> GPHMKHPLMNVWTLWYLENDRSKSWEDMQNEITSFDTVEDFWSLYNHIKPPSEIKLGSDYSLFKKNIRPMWEDAANKQGGRWVITLNKSSKTDLDNLWLDVLLCLIGEAFDHSDQICGAVINIRGKSNKISIWTADGNNEEAALEIGHKLR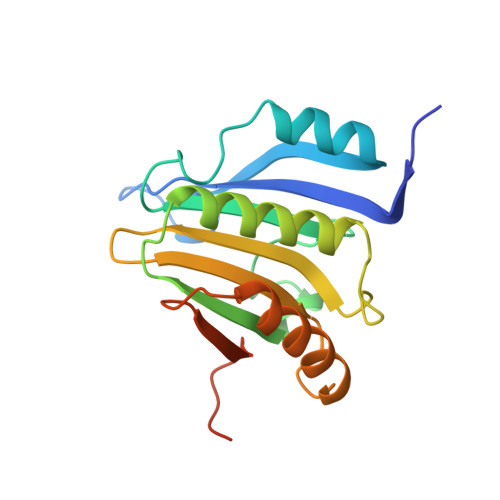DALRLGRNNSLQYQLHKDTMVKQGSNVKSIYTL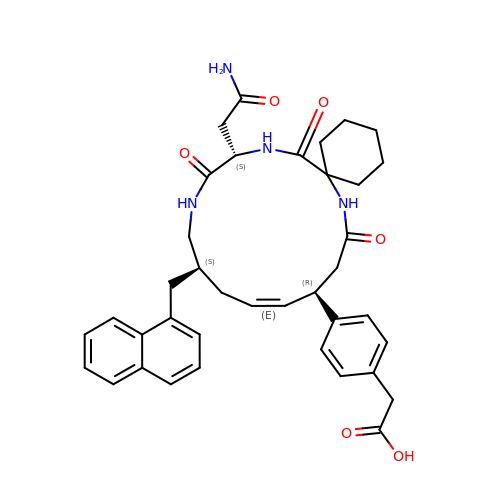(4-{(10R,11E,14S,18S)-18-(2-amino-2-oxoethyl)-14-[(naphthalen-1-yl)methyl]-8,17,20-trioxo-7,16,19-triazaspiro[5.14]icos-11-en-10-yl}phenyl)acetic acid | C38 H44 N4 O6 | ZYRZDVCTSBJOQD-GZNVFMSSSA-N>MTMDEQQSQAVAPVYVGGFLARYDQSPDEAELLLPRDVVEHWLHAQGQGQPSLSVALPLNINHDDTAVVGHVAAMQSVRDGLFCLGCVTSPRFLEIVRRASEKSELVSRGPVSPLQPDKVVEFLSGSYAGLSLSSRRCDDVEQATS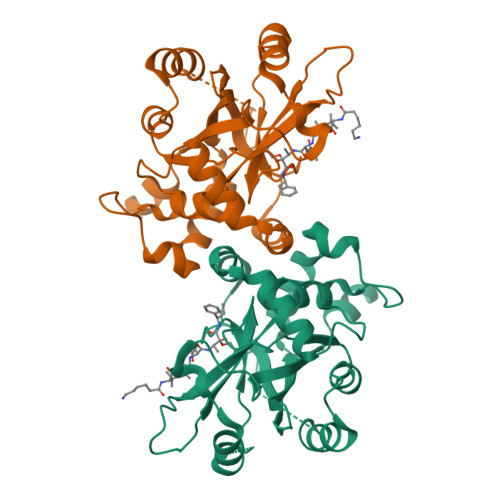LSGSETTPFKHVALCSVGRRRGTLAVYGRDPEWVTQRFPDLTAADRDGLRAQWQRCGSTAVDASGDPFRSDSYGLLGNSVDALYIRERLPKLRYDKQLVGVTERESYVKA[4x]> GPSSPMDVGELLSYQPNRGTKRPRDDEEEEQKMRRKQTGTRERGRYREEEMTVVEEADDDKKRLLQIIDRDGEEEEEEEEPLDESSVKKMILTFEKRSYKNQELRIKFPDNPEKFMESELDLNDIIQEMHVVATMPDLYHLLVELNAVQSLLGLLGHDNTDVSIAVVDLLQELTDIDTLHESEEGAEVLIDALVDGQVVALLVQNLERLDESVKEEADGVHNTLAIVENMAEFRPEMCTEGAQQGLLQWLLKRLKAKMPFDA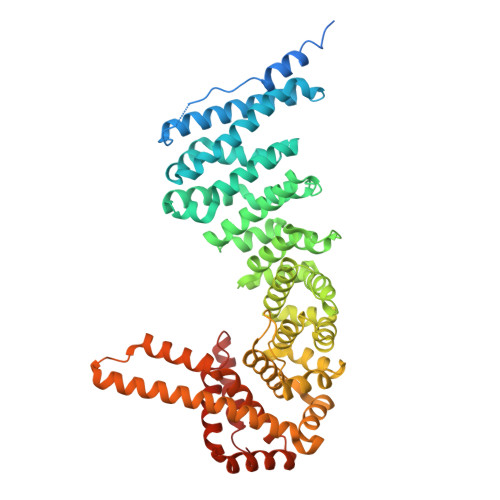NKLYCSEVLAILLQDNDENRELLGELDGIDVLLQQLSVFKRHNPSTAEEQEMMENLFDSLCSCLMLSSNRERFLKGEGLQLMNLMLREKKISRSSALKVLDHAMIGPEGTDNCHKFVDILGLRTIFPLFMKSPRKIKKVGTTEKEHEEHVCSILASLLRNLRGQQRTRLLNKFTENDSEKVDRLMELHFKYLGAMQVADKKIEGEKHDMVRRGEIIDNDTEEEFYLRRLDAGLFVLQHICYIMAEICNANVPQIRQRVHQILNMRGSSIKIVRHIIKEYAENIGDGRSPEFRENEQKRILGLLENF(2R)-1-[(2S)-2-methyl-3-sulfanyl-propanoyl]azepane-2-carboxylic 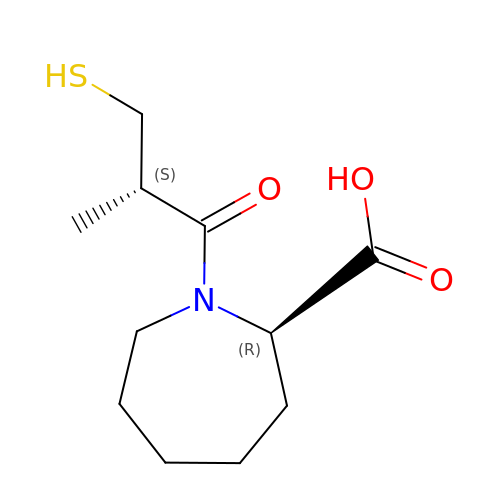acid | C11 H19 N O3 S | AKICLYTXRQJFDT-RKDXNWHRSA-N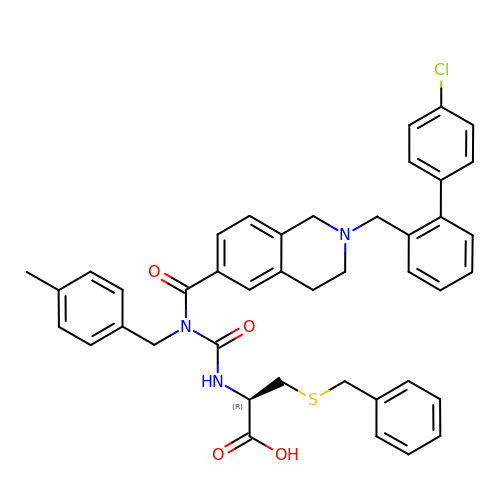(R)-3-(Benzylthio)-2-(3-(2-((4'-chloro-[1,1'-biphenyl]-2-yl)methyl)-1,2,3,4-tetrahydroisoquinoline-6-carbonyl)-3-(4-methylbenzyl)ureido)propanoic acid | C42 H40 Cl N3 O4 S | OFVMPKFGKDQYKS-KDXMTYKHSA-N SulE, an esterase, which detoxifies a variety of sulfonylurea herbicides through de-esterification, provides an attractive approach to remove environmental sulfonylurea herbicides and develop herbicide-tolerant crops. SulE catalyzes the de-esterification of a variety of sulfonylurea herbicides, such as MM, BM, SM, TM, TrM, EM, and CE, to the corresponding herbicidal-inactive parent acid. The structures show that SulE is a dimer with a lid loop in a domain-swapped β-hairpin covering the active site from the opposing monomer. SulE shows a similar catalytic triad consisting of Ser209, His333, and Glu232 at its active site.

To elucidate the catalytic mechanism of SulE, we solved the crystal structures of wild-type SulE in complex with CA, mutant S209A in complex with MM, and mutant S209A/H333A in complex with MM, SM, TM, TrM, EM, BM, and CE in the range of 1.29–1.63 Å. By contrast, the sulfonylurea bridge and the heterocyclic ring of MM was clearly observed and well localized to the active site of S209A/H333A, indicating that MM binds more stably in S209A/H333A than in S209A. Upon binding to SulE, the seven substrates adopted a similar conformation with a bend at the sulfonyl group, making the aromatic ring and heterocycle nearly perpendicular to each other. The side chain of residues Ala234, Phe257, Phe293, Trp296, Trp297 from subunit A and Ile43 from subunit B forms a deep hydrophobic pocket. The aromatic ring is trapped in the pocket and packed by Arg150 and Ala234 from both sides. However, the heterocycle moiety is located outside the pocket and only interacts with residues Ile43 and Phe257. The hydrophilic sulfonyl group is close to the hydrophilic area of the pocket and forms hydrogen bonds with one or both Arg150 and Tyr45. In the six structures of S209A/H333A bound to MM, EM, TrM, CE, SM, and BM, the ester O atom is hydrogen-bonded with the main chain nitrogen atoms of Gly78 and Ala210, forming an oxyanion hole. Superimposition of S209A/H333A-MM and P44R/S209A/H333A-MM complex structures revealed an outward movement of the lid loop from the active pocket. As compared with the MM bound to the S209A/H333A, the phenyl ring moiety of MM is located in a similar position, while the sulfonylurea bridge and heterocycle moiety undergo about 90° rotation, and the heterocycle occupied the position of Tyr45 side chain in apo structure.

>[2x]METDNVELAQSKRKVVLAEQGSFYIGGRTVTGPGKFDPSKPVIPYSNEGATFYINQMYVNFQAPVRPRGLPLVFWHGGGLTGHIWESTPDGRPGFQTLFVQDRHTVYTIDQPGRGRGNIPTFNGPFGQLEEESIVNTVTGNSSKEGAWVRDRLGPAPGQFFENSQFPRGYEDNYFKEMGFSPSISSDEIVDAVVKLVTHIGPCVLVTHAASGVLGMRVATHAKNVRGIVAYEPATSIFPKGKVPEIPPLADKKSQIFPPFEIQESYFKKLAKIPIQFVFGDNIPKNPKSAYWFLDWWRVTRYAHSLSLEAINKLGGQASLLDLPTAGLRGNTAFPFTDRNNVQVASLLSDFLGKHGLDQNESLEHHHHHH1-(cyclopropylmethyl)-2,5-dimethyl-pyrrole-3-carboxylic acid | C11 H15 N O2 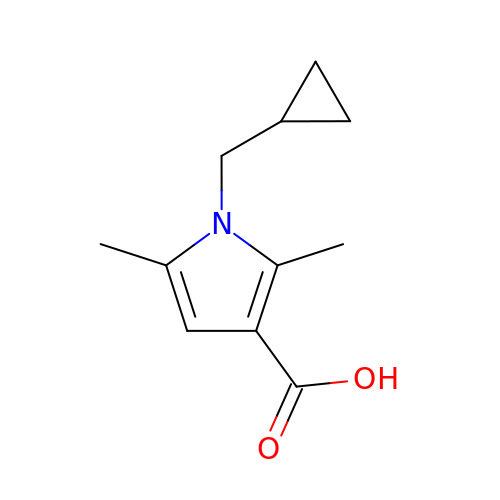| IRPSDSAYDMWHCN-UHFFFAOYSA-N> GSHMASMSKDEVKREAKDTDGNPEIKGERRRLHSE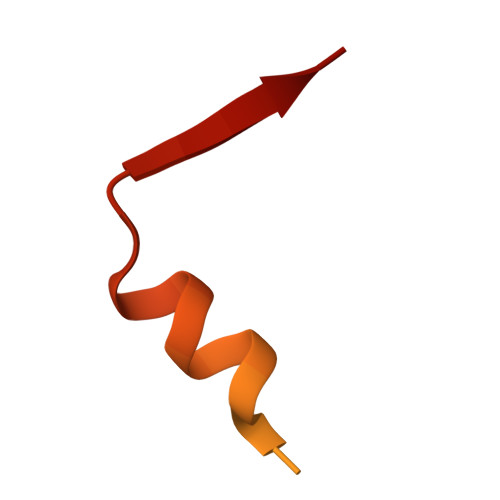IQSGSLANNIKKSTVIVKN>AHHHHHHGHHHQLVKKVLLINGPNLNLLGTREPEKYGTTSLSDIEQAAIEQAKLKNNDSEVLVFQSNTEGFIIDRIHEAKRQGVGFVVINAGAYTHTSVGIRDALLGTAIPFIEVHITNVHQREPFRHQSYLSDKAVAVICGLGVYGYTAAIEYALNYQLDGDLEAA[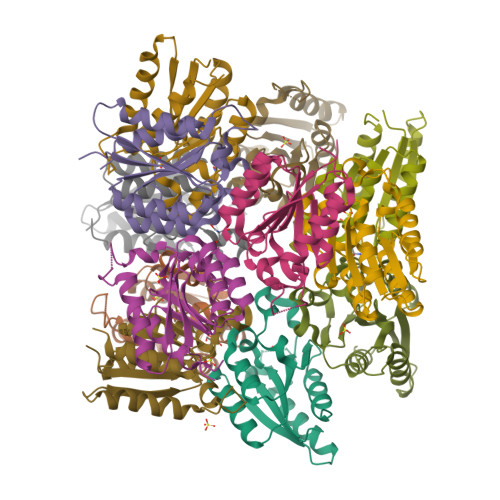24x]> STTEVVMENVTAFWEEGFGELFEKAKQNNNNRKTSNGDDSLSFSNFSLLGTPVLKDINFKIERGQLLAVAGSTGAGKTSLLMMIMGELEPSEGKIKHSGRISFCS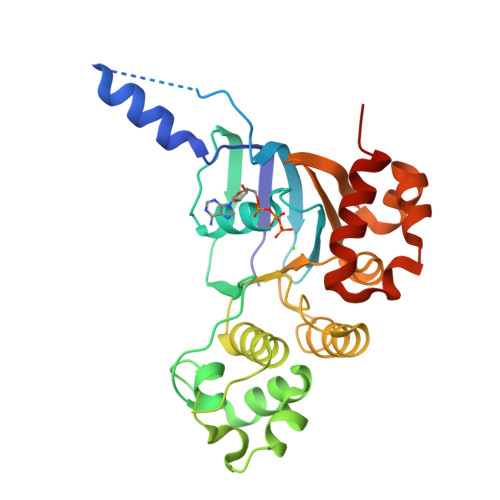QNSWIMPGTIKENIIGVSYDEYRYRSVIKACQLEEDISKFAEKDNIVLGEGGITLSGGQRARISLARAVYKDADLYLLDSPFGYLDVLTEKEIFESCVCKLMANKTRILVTSKMEHLKKADKILILHEGSSYFYGTFSELQNLRPDFSSKLMGCDSFDQFSAERRNSILTETLHRFSLEGDAPVS Bacterial cells use several evolutionarily-distinct genome segregation systems, the most common of which is the type I Par system. It consists of an adapter protein, ParB, that binds to the DNA cargo via interaction with the parS DNA sequence; and an ATPase, ParA, that binds nonspecific DNA and mediates cargo transport. Each chromosome encodes its own segregation complex, with Chr1 encoding a chromosomal type Ib system, and Chr2 encoding a plasmid-like type Ia system. In this study, we have reported the structure of the ParA2vc protein, in three states: apo, nucleotide-bound (ADP) and in a filamentous complex with nucleotide and DNA.

As indicated, the presence of slowly hydrolysable ATP analogue was required to obtain stable filaments, suitable for cryo-EM analysis. Using this data, we were able to obtain a map to 4.5 Å resolution, by helical reconstruction. ParA2vc forms a left-handed helix, with a rise of 28.68 Å and a twist of −80.57°. Density for the ATPγS and Mg molecules is also clearly delineated in the active site. Our structure of the ParA2vc-DNA filament reveals that each ParA2vc molecule binds to DNA via two interaction sites: (1) In the central ParA domain, three regions (residues 322–328, 345–353, and 376–382) interact with the DNA backbone. (2) In the N-terminal winged helix-turn-helix domain, the loop between residues 74 and 80 is inserted deep into the minor groove. In the structure of the ParA2vc-DNA filament reported here, adjacent ParA dimers form extensive contacts, with a surface area of ~1500 Å2. This interface is largely mediated by three regions: two helices, located at the C-terminus (residues 325–339 and 381–405), and a helix-turn-helix motif from the N-terminal domain, forming electrostatic contacts. Specifically, helix 1 undergoes a striking conformational change, merging with helix 2 to form a single, extended helix ~15 Å from its position in the structures obtained without DNA. Helix 1 forms a cross-dimer interaction, in the ParA2vc dimer. As a consequence, the angle between the two molecules in the filament structure is altered by ~30 degrees, compared to the crystal structures described above.

>MAMKREQTIENLYQLAQLTQQVQADRIEIVLEERRDEHFPPMSKALMETRSGLTRRKLDEAIAKMEEAGHQFTKNNANHYSISLSEAHMLMDAAGVPKFHERKKNNENKPWIINVQNQKGGTGKSMTAVHLAACLALNLDKRYRICLIDLDPQGSLRLFLNPQISLAEHTNIYSAVDIMLDNVPDGVQVDTEFLRKNVMLPTQYPNLKTISAFPEDAMFNAEAWQYLSQNQSLDIVRLLKEKLIDKIASDFDIIMIDTGPHVDPLVWNAMYASNALLIPCAAKRLDWASTVNFFQHLPTVYEMFPEDWKGLEFVRLMPTMFEDDNKKQVSVLTEMNYLLGDQVMMATIPRSRAFETCADTYSTVFDLTVNDFEGGKKTLATAQDAVQKSALELERVLHSHWSSLNQG[8x]> WIAQELRLIGDL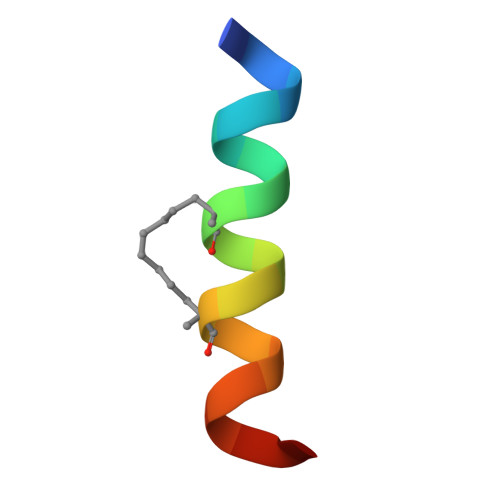FNAYYAX> EERKKELAKEVIETAKKLIEK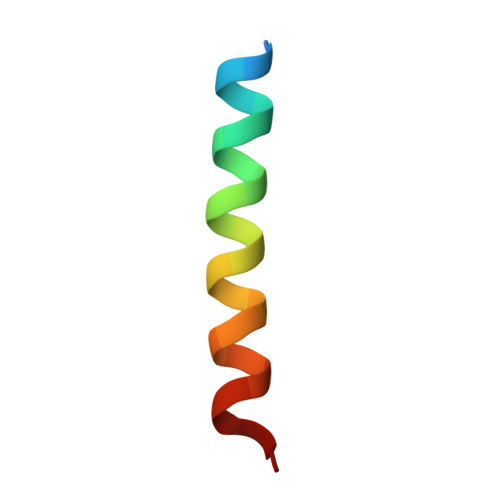LAKEE>GMEKPTNYSQETIASIAQKYQKLAEDINKDRKNNIADQTVIYLLSESLSDPDRVSNVTVSHDVLPNIKAIKNSTTAGLMQSDSYGGGTANMEFQTLTSLPFYNFSSSVSVLYSEVFPKMAKPHTISEFYQGKNRIAMHPASANNFNRKTVYSNLGFSKFLALSGSKDKFKNIENVGLLTSDKTVYNNILSLINPSESQFFSVITMQNHIPWSSDYPEEIVAEGKNFTEEENHNLTSYARLLSFTDKETRAFLEKLTQINKPITVVFYGD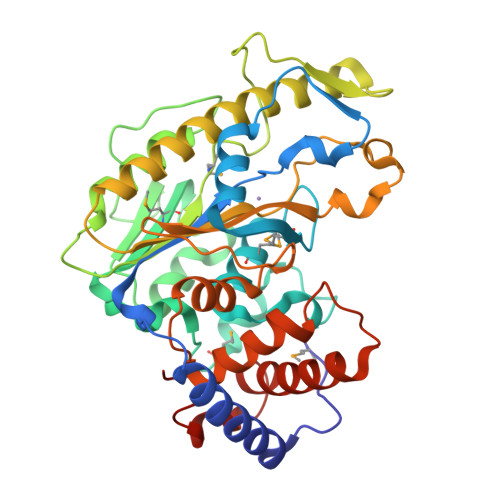HLPGLYPDSAFNKHIENKYLTDYFIWSNGTNEKKNHPLINSSDFTAALFEHTDSKVSPYYALLTEVLNKASVDKSPDSPEVKAIQNDLKNIQYDVTIGKGYLLKHKTFFKISR[2x]> MFERFTDRARRV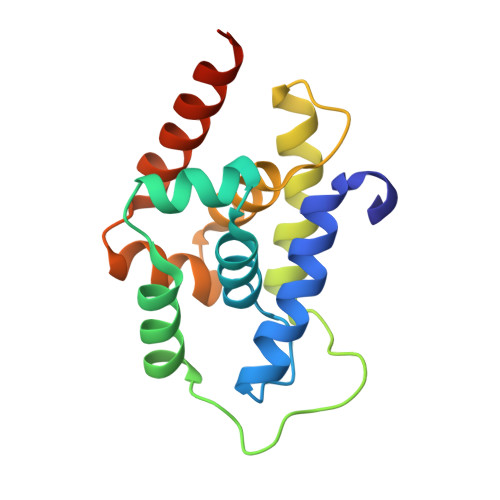VVLAQEEARMLNHNYIGTEHILLGLIHEGEGVAAKSLESLGISLEGVRSQVEEIIGQGQQAPSGHIPYTPRAKKVLELSLREALQLGHNYIGTEHILLGLIREGEGVAAQVLVKLGAELTRVRQQVIQLLSGYLEHHHHHH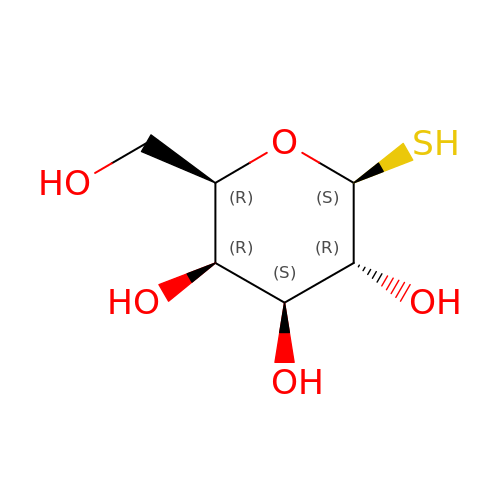1-thio-beta-D-galactopyranose | C6 H12 O5 S | JUSMHIGDXPKSID-PHYPRBDBSA-N> MDYKDDDDKMPSPTTVPVATAGRLAEPYIDPAAQVHAIASIIGDVRIAAGVRVAAGVSIRADEGAPFQVGKESILQEGAVIHGLEYGRVLGDDQADYSVWIGQRVAITHKALIHGPAYLGDDCFVGFRSTVFNAR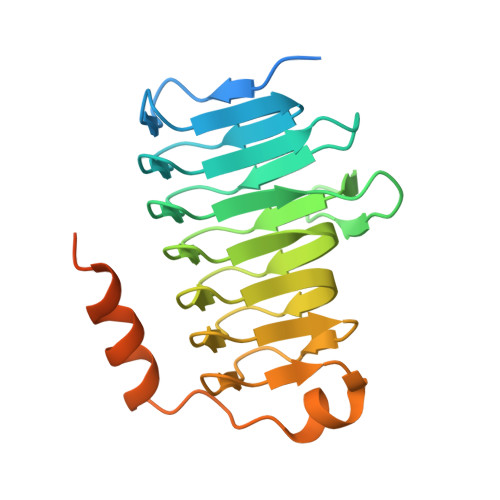VGAGSVIMMHALVQDVEIPPGRYVPSGAIITTQQQADRLPEVRPEDREFARHIIGSPPVIVRSTPAATADFHSTPTPSPLRPS To generalize this engineering approach for crystal contacts, a non-ADH-homologous enzyme was selected to apply the established strategies to the Nostoc sp. PCC 1720 ene reductase (NostocER). This oxidoreductase from the old yellow enzyme family (OYE, EC 1.6.99.1) catalyzes the trans-hydrogenations of activated alkenes, demonstrating its industrial relevance as a biocatalyst. As OYEs are strongly dependent on cost-intensive NADPH as a cofactor, Mähler et al. engineered NADH-accepting variants (NostocER1) by exchanging NostocER loop regions at cofactor-binding sites to ER loop regions from Achromobacter sp. JA81 and Acaryochloris marina with a higher NADH affinity. For this study, the NostocER1 Loop1,5 variant (NostocER1-L1,5) was selected as an example protein for the rational introduction of Lys–Glu interactions at crystal contacts to demonstrate the impact of rational single amino acid exchanges on the crystallizability of proteins and enhance protein crystallization.

Mutant Q350K crystallized similarly to the WT regarding crystal size and amount. Mutants Q204K and Q350K crystallized in space group P212121, with the RMSD of the crystalline environment in this crystal packing indicating structural differences. However, as demonstrated by Figure 8, the crystal contacts at the mutation sites were present as derived from the NspER1-L1,5 wild-type structure. The crystal contact at positions Q204K and Q350K both reveal an approximation of the intermolecular partners E89 (5.3 Å) and E27 (7.8 Å), respectively, compared to the WT. For mutants Q204K (4.5 Å) and Q350K (7.8 Å), the formation of a long-range ion pair between Lys–Glu, which could exhibit an interaction within a range of 5–10 Å, could account for the enhanced crystallizability, especially for mutant Q204K. Introducing a lysine at any of the neighboring NspER1-L1,5 positions Q350, (D352), and T354 led to an interaction with the intermolecular amino acid residue of E25/27. The neighboring NspER1-L1,5 mutants Q350K, D352K, and T354K led to an interaction with intermolecular E25/27 and an increase in crystallizability (Section 3.2, Section 3.3 and Section 3.4), with the strongest impact for T354K.

> MGHHHHHHGSGSTNINLFSSYQLGELELPNRIVMAPLTRSRAGEGNVPHQLNAIYYGQRASAGLIIAEATQVTPQGQGYPHTPGIHSPEQVAGWKLVTDTVHQQGGRIFLQLWHVGRISHPDLQPDGGLPVAPSAIAPKGEVLTYEGKKPYVTPRALDTSEIPAIVEQYRQGAANALAAGFDGVEIHAANGYLIDQFLRDGTNQRTDEYGGAIENRARLLLEVTEAITSVWDSQRVGVRLSPLTTLNGCVDSHPLETFGYVAQALNRFNLSYLHIFEAIDADIRHGGTVVPTSHLRDRFTGTLIVNGGYTREKGDTVIANKAADLVAFGTLFISNPDLPERLEVNAPLNKADPTTFYGGGEKGYTDYPFLAVANK>[4x]GMRPALYFCGSIRGGREDRTLYERIVSRLRRFGTVLTEHVAAAELGARGEEAAGGDRLIHEQDLEWLQQADVVVAEVTQPSLGVGYELGRAVAFNKRILCLFRPQSGRVL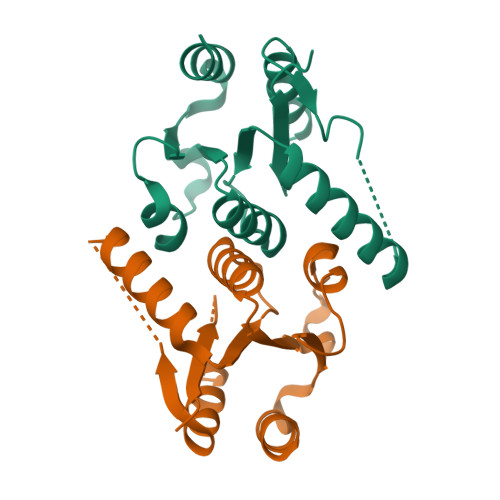SAMIRGAADGSRFQVWDYEEGEVEALLDRYFEADP> MKEFYLTVEQIGDSIFERYIDSNGRERTREVEYKPSLFAHCPESQA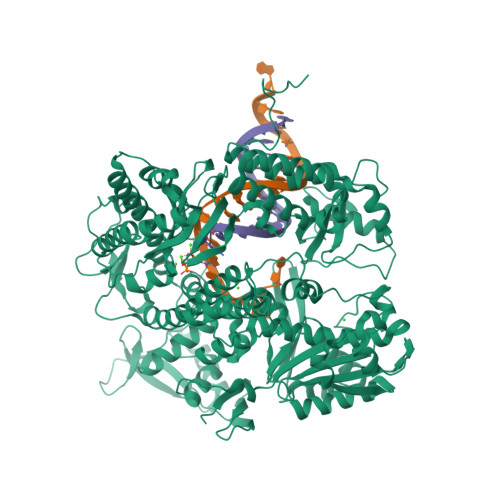TKYFDIYGKPCTRKLFANMRDASQWIKRMEDIGLEALGMDDFKLAYLSDTYNYEIKYDHTKIRVANFDIEVTSPDGFPEPSQAKHPIDAITHYDSIDDRFYVFDLLNSPYGNVEEWSIEIAAKLQEQGGDEVPSEIIDKIIYMPFDNEKELLMEYLNFWQQKTPVILTGWNVESFAIPYVYNRIKNIFGESTAKRLSPHRKTRVKVIENMYGSREIITLFGISVLDYIDLYKKFSFTNQPSYSLDYISEFELNVGKLKYDGPISKLRESNHQRYISYNIIAVYRVLQIDAKRQFINLSLDMGYYAKIQIQSVFSPIKTWDAIIFNSLKEQNKVIPQGRSHPVQPYPGAFVKEPIPNRYKYVMSFDLTSLYPSIIRQVNISPETIAGTFKVAPLHDYINAVAERPSDVYSCSPNGMMYYKDRDGVVPTEITKVFNQRKEHKGYMLAAQRNGEIIKEALHNPNLSVDEPLDVDYRFDFSDEIKEKIKKLSAKSLNEMLFRAQRTEVAGMTAQINRKLLINGLAGALGNVWFRYYDLRNATAITTFGQMALQWIERKVNEYLNEVCGTEGEAFVLYGDTDSIYVSADKIIDKVGESKFRDTNHWVDFLDKFARERMEPAIDRGFREMCEYMNNKQHLMFMDREAIAGPPLGSKGIGGFWTGKKRYALNVWDMEGTRYAEPKLKIMGLETQKSSTPKAVQKALKECIRRMLQEGEESLQEYFKEFEKEFRQLNYISIASVSSANNIAKYDVGGFPGPKCPFHIRGILTYNRAIKGNIDAPQVVEGEKVYVLPLREGNPFGDKCIAWPSGTEITDLIKDDVLHWMDYTVLLEKTFIKPLEGFTSAAKLDYEKKASLFDMFDF> GHTYFGIDYQYYRDFAENKGKFTVGAQNIKVYNKQGQLVGTSMTKAPMIDFSVVSRNGVAALVENQYIVSVAHNVGYTDVDFGAEGNNPDQHRFTYKIV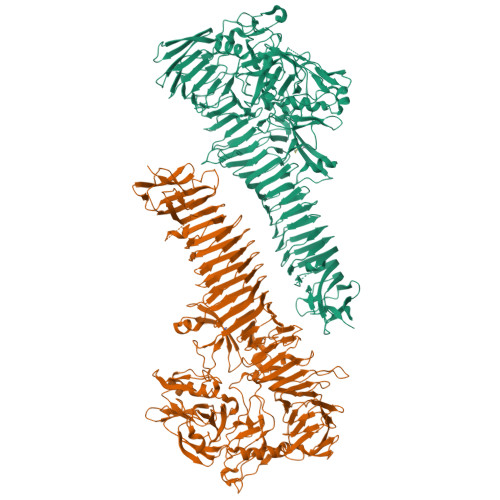KRNNYKKDNLHPYEDDYHNPRLHKFVTEAAPIDMTSNMNGSTYSDRTKYPERVRIGSGRQFWRNDQDKGDQVAGAYHYLTAGNTHNQRGAGNGYSYLGGDVRKAGEYGPLPIAGSKGDSGSPMFIYDAEKQKWLINGILREGNPFEGKENGFQLVRKSYFDEIFERDLHTSLYTRAGNGVYTISGNDNGQGSITQKSGIPSEIKITLANMSLPLKEKDKVHNPRYDGPNIYSPRLNNGETLYFMDQKQGSLIFASDINQGAGGLYFEGNFTVSPNSNQTWQGAGIHVSENSTVTWKVNGVEHDRLSKIGKGTLHVQAKGENKGSISVGDGKVILEQQADDQGNKQAFSEIGLVSGRGTVQLNDDKQFDTDKFYFGFRGGRLDLNGHSLTFKRIQNTDEGAMIVNHNTTQAANVTITGNESIVLPNGNNINKLDYRKEIAYNGWFGETDKNKHNGRLNLIYKPTTEDRTLLLSGGTNLKGDITQTKGKLFFSGRPTPHAYNHLNKRWSEMEGIPQGEIVWDHDWINRTFKAENFQIKGGSAVVSRNVSSIEGNWTVSNNANATFGVVPNQQNTICTRSDWTGLTTCQKVDLTDTKVINSIPKTQINGSINLTDNATANVKGLAKLNGNVTLTNHSQFTLSNNATQIGNIRLSDNSTATVDNANLNGNVHLTDSAQFSLKNSHFSHQIQGDKGTTVTLENATWTMPSDTTLQNLTLNNSTITLNSAYSASSNNTPRRRSLETETTPTSAEHRFNTLTVNGKLSGQGTFQFTSSLFGYKSDKLKLSNDAEGDYILSVRNTGKEPETLEQLTLVESKDNQPLSDKLKFTLENDHVDAGALRYKLVKNDGEFRLHNPIKEQELHNDLVRAEQAERTLEAKQVEPTAKTQTGEPKVRSRRAARAAFPDTLPDQSLLNA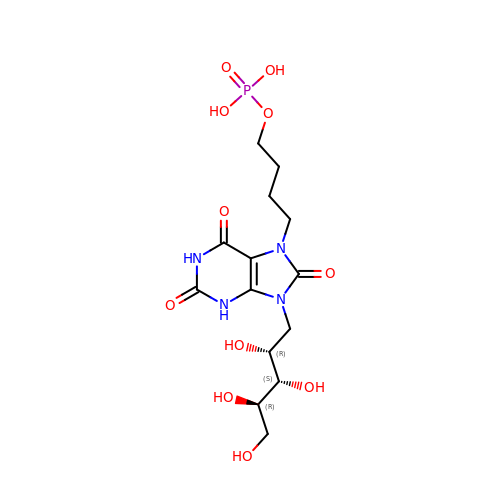4-{2,6,8-TRIOXO-9-[(2R,3S,4R)-2,3,4,5-TETRAHYDROXYPENTYL]-1,2,3,6,8,9-HEXAHYDRO-7H-PURIN-7-YL}BUTYL DIHYDROGEN PHOSPHATE | C14 H23 N4 O11 P | VBXZSBKAJFXURR-MRTMQBJTSA-N> MSKDLVHPSLIRAGIVELEMAEETTDLINRTIESNQAHLQGEPLYVDSLPEDMSRLRIEDKSRRTKTEEEERDEGSSEEDNYLSEGQDPLIPFQNFLDEIGARAVKRLKTG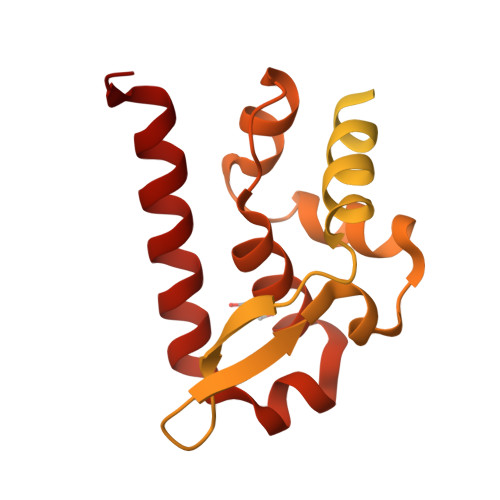EGFFRVWSALSDDIKGYVSTNIMTSGERDTKSIQIQTEPTASVSSGNESRHDSESMHDPNDKKDHTPDHDVVPDIESSTDKGEIRDIEGEVAHQVAESFSKKYKFPSRSSGIFLWNFEQLKMNLDDIVKAAMNVPGVERIAEKGGKLPLRCILGFVALDSSKRFRLLADNDKVARLIQEDINSYMARLEEAE>MALSAEGSSGGSRGGSPKAEAASVPSWPQILGRLTDNRDLARGQAAWAMDQIMTGNARPAQIAAFAVAMTMKAPTADEVGELAGVMLSHAHPLPADTVPDDAVDVVGTGGDGVNTVNLSTMAAIVVAAAGVPVVKHGNRAASSLSGGADTLEALGVRIDLGPDLVARSLAEVGIGFCFAARFHPSYRHAAAVRREIGVPTVFNLLGPLTNPARPRAGLIGCAFADLAEVMAGVFAARRSSVLVVHGDDGLDELTTTTTSTIWRVAAGSVDKLTFDPAGFGFARAQLDQLAGGDAQAN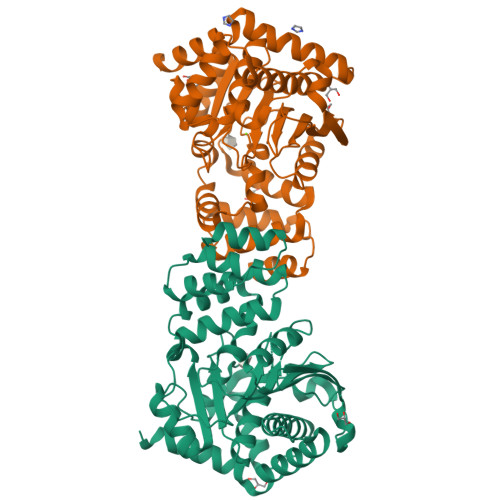AAAVRAVLGGARGPVRDAVVLNAAGAIVAHAGLSSRAEWLPAWEEGLRRASAAIDTGAAEQLLARWVRFGRQILEHHHHHH[2x]> MAGSGSERAEHQIILPESHLSSPLVKHKLLYYWKLTGLPLPDECDFDHLILSRQWKKILESSTPDIERMIKLGRSVHQTLSHSSKLTGILHPRCLEDLVGLDIPDSTNKFRRIEKKIQIHNTRYGEPF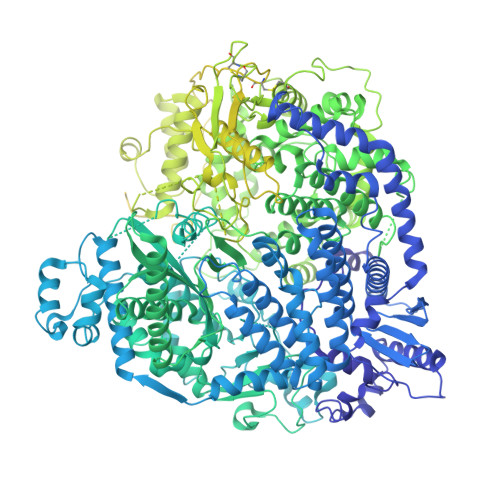TRLCSYVEKKLLGSSWTHKIRRSEEFDSLRTDPAFWFHSSWSTAKFAWLHVKQIQRHLIVAARTRSASNKLVTLSHRSGQVFITPELVIVTHTNENKFTCLSQELVLMYADMMEGRDMVNIISSTAVHLRCLAEKIDDILRLVDALARDLGNQVYDVVALMEGFAYGAVQLLEPSGTFAGDFFSFNLQELRDTLICLLPQRIADSVTHAIANIFSGLEQNQAAEMLCLLRLWGHPLLESRAAAKAVRAQMCAPKMVDFDMILQVLSFFKGTIINGYRKKNAGVWPRVKAHTIYGNVIAQLHADSAEISHDIMLREYKNLSAIEFEACIEYDPVTNLSMFLKDKAIAHPRNNWLASFRRNLLSEEQKKNVQDSTSTNRLLIEFLESNDFDPYKEMEYLTTLEYLRDDSVAVSYSLKEEEVKVNGRIFAKLTKKLRNCQVMAEGILADQIAPFFQGNGVIQDSISLTKSMLAMSQLSYNSNRKRITDCKERVSSSRNHDLKGKHRRRVATFITTDLQKYCLNWRYQTIKLFAHAINQLMGLPHFFEWIHLRLMDTTMFVGDPFNPPSDPTDYDLTKVPNDDIYIVSARGGIEGLCQKLWTMISIAAIQLAAARSHCRVACMVQGDNQVIAVTREVRPDDSPESVLTQLHEASDNFFRELIHVNHLIGHNLKDRETIRSDTFFIYSKRIFKDGAILSQVLKNSSKLVLVSGDLSENTVMSCANISSTVARLCENGLPKDFCYYLNYLMSCIQTYFDSEFSITSSTQSGSNQSWINDIPFIHSYVLTPAQLGGLSNLQYSRLYTRNIGDPGTTAFAEVKRLEAVGLLGPNIMTNILTRPPGNGDWASLCNDPYSFNFESVASPSIVLKKHTQRVLFETCSNPLLSGVHTEDNEAEEKALAEYLLNQEVIHPRVAHAIMEASSVGRRKQIQGLVDTTNTVIKIALSRKPLGIKRLARIINYSSMHAMLFRDDVFLSNRANHPLVSSDMCSLALADYARNRSWSPLTGGRKILGVSNPDTIELVEGEILSISGGCSKCDSGDEQFTWFHLPSNIELTDDTSKNPPMRVPYLGSKTQERRAASLAKIAHMSPHVKAALRASSVLIWAYGDNDINWTAALKLARSRCNISSEYLRLLSPLPTAGNLQHRLDDGITQMTFTPASLYRVSPYVHISNDSQRLFTEEGVKEGNVVYQQIMLLGLSLIESLFPMTVTKTYDEITLHLHSKFSCCIREAPVAVPFELTGVAPDLRVVASNKFMYDPNPVAEGDFARLDLAIFKSYELNLESYSTVELMNILSISSGKLIGQSVVSYDEETSIKNDAIIVYDNTRNWISEAQNSDVVRLFEYAALEVLLDCSYQLYYLRVRGLNNVVLYMSDLYKNMPGILLSNIAATISHPIIHSRLHTVGLISHDGSHQLADTDFIELSAKLLVSCTRRVVSGLYAGNKYDLLFPSVLDDNLNEKMLQLISRLCCLYTVLFATTREIPKIRGLPAEEKCAMLTEYLLSDAVRPLLSPEQVDSITSPSIVTFPANLYYMSRKSLNLIREREDRDSILALMFPQEPLFEFPLVQDIGARVKDQLTMKPAAFLHELDLSAPARYDAYTLEQARSDCALADMGEDQLVRYLFRGVGTASSSWYKASHLLSVPEIRCARHGNSLYLAEGSGAIMSLLELHIPHETIYYNTLFSNEMNPPQRHFGPTPTQFLNSVVYRNLQAEVPCKDGFVQEFRTLWRENTEESDLTSDKAVGYITSVVPYRSVSLLHCDIEIPPGSNQSLLDQLATNLSLIAMHSVREGGVVIVKILYSMGYYFHLLVNLFTPCSVKGYVLSNGYACRGDMECYVVFVMGYLGGPTFVNEVVRMAKTLIQRHGTLLAKSDETALMALFTSQKQRVDNILSSPLPRLAKLLRRNIDTALIEAGGQPVRPFCAESLVNTLSDITQTTQVIASHIDTVIRSVIYMEAEGDLADTVFLFTPYNLSIDGKKRTSLKQCTRQILEVTILGLGPEDLNRVGDIISLILRGTISLEDLIPLRTYLKMSTCPKYLKSVLGLTKLREMFSDGSMLYLTRAQQKFYMKTVGNAVKGYYNSSKNENLYFQG> LPSGSDPAFSQPKSVLDAGLTCQGASPSSVSKPILLVPGTGTTGPQSFDSNWIPLSTQLGYTPCWISPPPFMLNDTQVNTEYMVNAITALYAGSGNNKLPVLTWSQGGLVAQWGLTFFPSIRSKVDRLMAFAPDYKGTVLAGPLDALAVSAPSVWQQTTGSALTTALRNAGGLTQIVPTTNLYSATDEIVQPQVSNSPLDSSYLFNGKNVQAQAVCGPLFVIDHAGSLTSQFSYVVGRSALRSTTGQARSADYGITDCNPLPANDLTPEQKVAAAALLAPAAAAIVAGPKQNCEPDLMPYARPFAVGKRTC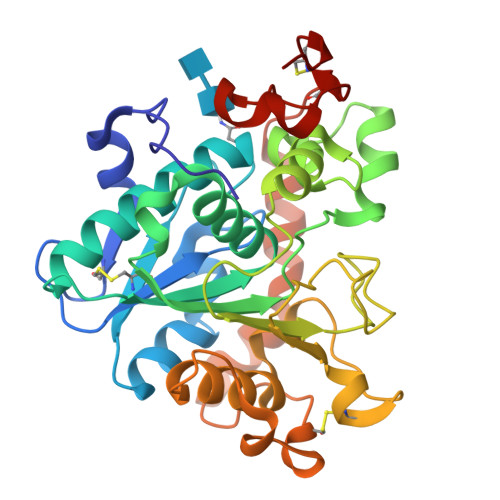SGIVTP>MEVYYTSLRCRCVQES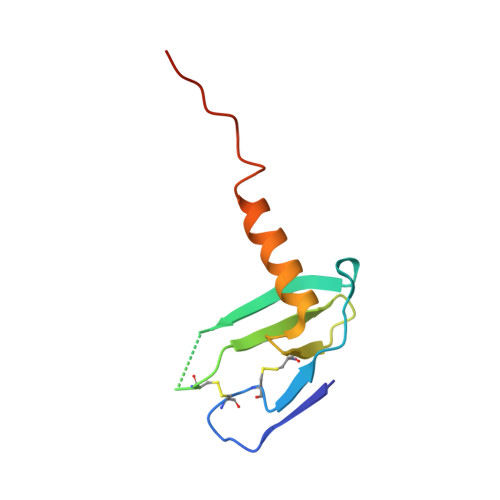SVFIPRRFIDRIQILPRGNGCPRKEIIVWKKNKSIVCVDPQAEWIQRMMEVLRKRSSSTLPVPVFKRKIP[7x]> PISPIETVPVKLKPGMD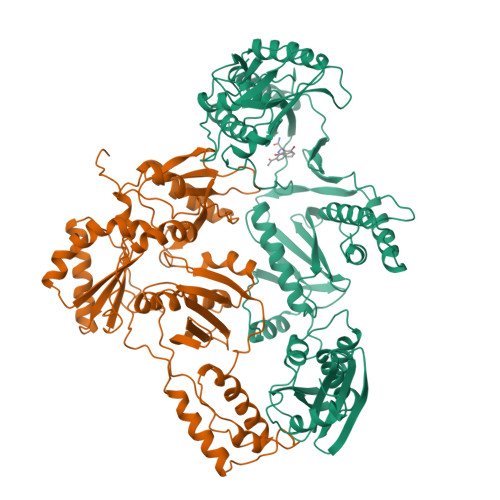GPKVKQWPLTEEKIKALVEICTEMEKEGKISKIGPENPYNTPVFAIKKKDSTKWRKLVDFRELNKRTQDFWEVQLGIPHPAGLKKKKSVTVLDVGDAYFSVPLDEDFRKYTAFTIPSINNETPGIRYQYNVLPQGWKGSPAIFQSSMTKILEPFKKQNPDIVIYQYMDDLYVGSDLEIGQHRTKIEELRQHLLRWGLTTPDKKHQKEPPFLWMGYELHPDKWTVQPIVLPEKDSWTVNDIQKLVGKLNWASQIYPGIKVRQLSKLLRGTKALTEVIPLTEEAELELAENREILKEPVHGVYYDPSKDLIAEIQKQGQGQWTYQIYQEPFKNLKTGKYARMRGAHTNDVKQLTEAVQKITTESIVIWGKTPKFKLPIQKETWETWWTEYWQATWIPEWEFVNTPPLVKLWYQLEKEPIVGAETFYVDGAANRETKLGKAGYVTNKGRQKVVPLTNTTNQKTELQAIYLALQDSGLEVNIVTDSQYALGIIQAQPDKSESELVNQIIEQLIKKEKVYLAWVPAHKGIGGNEQVDKLVSAGIRK;> PISPIETVPVKLKPGMDGPKVKQWPLTEEKIKALVEICTEMEKEGKISKIGPENPYNTPVFAIKKKDSTKWRKLVDFRELNKRTQDFWEVQLGIPHPAGLKKKKSVTVLDVGDAYFSVPLDEDFRKYTAFTIPSINNETPGIRYQYNVLPQGWKGSPAIFQSSMTKILEPFRKQNPDIVIYQYMDDLYVGSDLEIGQHRTKIEELRQHLLRWGLTTPDKKHQKEPPFLWMGYELHPDKWTVQPIVLPEKDSWTVNDIQKLVGKLNWASQIYPGIKVRQLSKLLRGTKALTEVIPLTEEAELELAENREILKEPVHGVYYDPSKDLIAEIQKQGQGQWTYQIYQEPFKNLKTGKYARTRGAHTNDVKQLTEAVQKITTESIVIWGKTPKFKLPIQKETWETWWTEYWQATWIPEWEFVNTPPLVKLWY>[2x]CG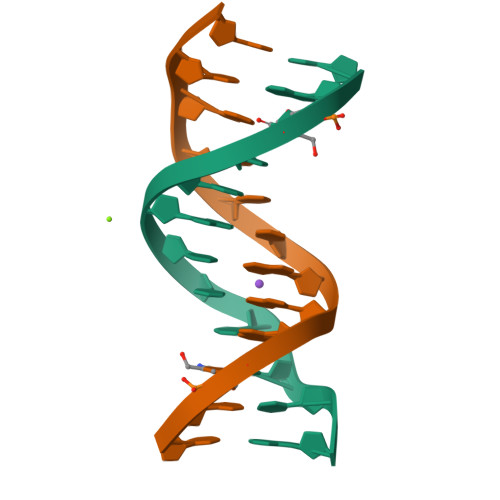XGAATTCGCG>[2x]SDKIIHLTDDSFDEVIRNNKLILVDFWAEWCGPCKMIAPILDEIADEYQGKLTVAKL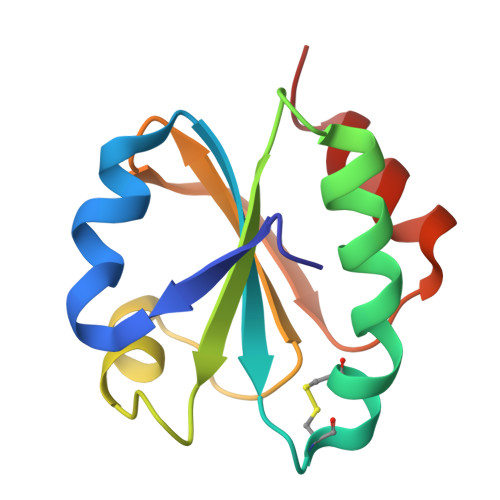NIDQNPGTAPKYGIRGIPTLLLFKNGEVAATKVGALSKGQLKEFLDANLA5-ethyl-5-[(2S)-pentan-2-yl]pyrimidine-2,4,6(1H,3H,5H)-trione | C11 H18 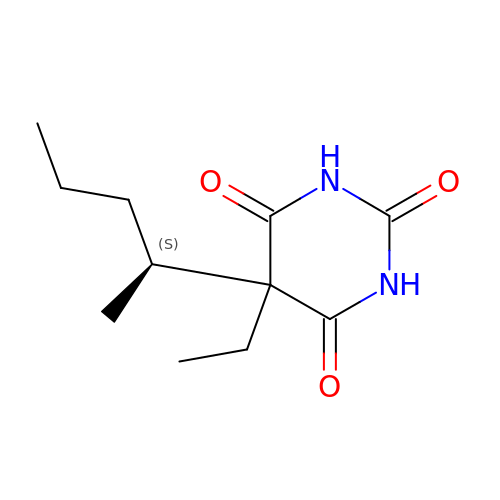N2 O3 | WEXRUCMBJFQVBZ-ZETCQYMHSA-N>[5x]GAMNEAVKTLDGWFCLHDFRSIDWAAWRELNPGNQELMLNELSHFLSDMEITKNIGEGEHTIYSILGQKADLVFFTLRDSLEALNEVENRFNKLAIADYLLPTYSYISVVELSNYLASHMAGGDDPYQNKGVRARLYPALPPKKHICFYP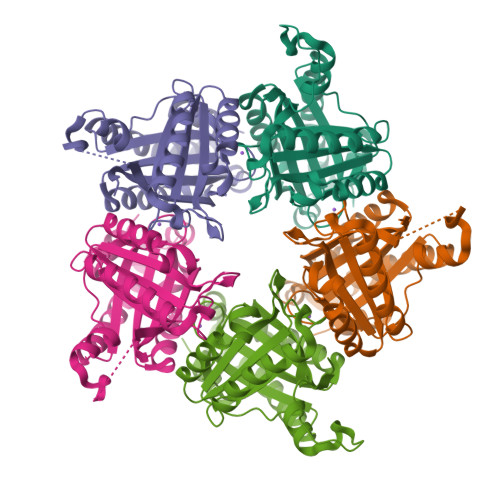MSKKRDGADNWYMLPMEERQQLIRDHGLIGRSYAGKVQQIIGGSIGFDDYEWGVTLFSDDALEFKRIVTEMRFDEASARYAEFGSFFIGNLLLSEQLSKLFTI(2S)-2-({(3R)-3-[4-amino-3-(4-phenoxyphenyl)-1H-pyrazolo[3,4-d]pyrimidin-1-yl]piperidin-1-yl}carbonyl)-4,4-dimethylpentanenitrile | C30 H33 N7 O2 | 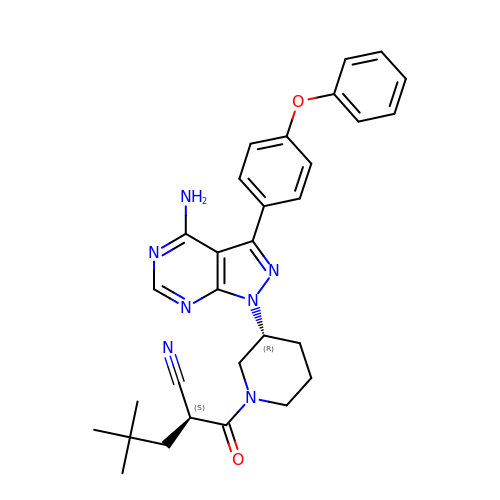DZSBLWYJPNCWLI-FGZHOGPDSA-N> QDTSPDTLVCTANRFEQPRSTVLAPTTVVTRQDIDRWQSTSVNDVLRRLPGVDITQNGGSGQLSSIFIRGTNASHVLVLIDGVRLNLAGVSGSADLSQFPIALVQRVEYIRGPRSAVYGSDAIGGVVNIITTRDEPGTEISAGWGSNSYQNYDVSTQQQLGDKTRVTLLGDYAHTHGYDVVAYGNTGTQAQTDNDGFLSKTLYGALEHNFTDAWSGFVRGY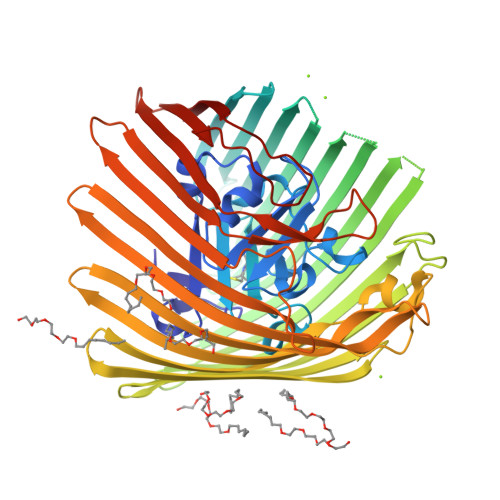GYDNRTNYDAYYSPGSPLLDTRKLYSQSWDAGLRYNGELIKSQLITSYSHSKDYNYDPHYGRYDSSATLDEMKQYTVQWANNVIVGHGSIGAGVDWQKQTTTPGTGYVEDGYDQRNTGIYLTGLQQVGDFTFEGAARSDDNSQFGRHGTWQTSAGWEFIEGYRFIASYGTSYKAPNLGQLYGFYGNPNLDPEKSKQWEGAFEGLTAGVNWRISGYRNDVSDLIDYDDHTLKYYNEGKARIKGVEATANFDTGPLTHTVSYDYVDARNAITDTPLLRRAKQQVKYQLDWQLYDFDWGITYQYLGTRYDKDYSSYPYQTVKMGGVSLWDLAVAYPVTSHLTVRGKIANLFDKDYETVYGYQTAGREYTLSGSYTF1H-benzotriazole | C6 H5 N3 | 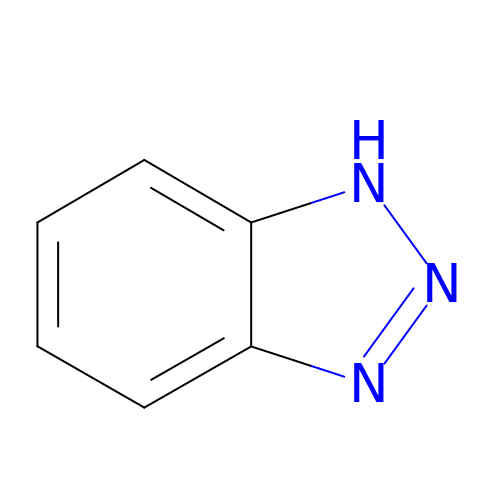QRUDEWIWKLJBPS-UHFFFAOYSA-N> MTQVAKKILVTCALPYANGSIHLGHMLEHIQADVWVRYQRMRGHEVNFICADDAHGTPIMLKAQQLGITPEQMIGEMSQEHQTDFAGFNISYDNYHSTHSEENRQLSELIYSRLKENGFIKNRTISQLYDPEKGMFLPDRFVKGTCPKCKSPDQYGDNCEVCGATYSPTELIEPKSVVSGATPVMRDSEHFFFDLPSFSEMLQAWTRSGALQEQVANKMQEWFESGLQQWDISRDAPYFGFEIPNAPGKYFYVWLDAPIGYMGSFKNLCDKRGDSVSFDEYWKKDSTAELYHFIGKDIVYFHSLFWPAMLEGSNFRKPSNLFVHGYVTVNGAKMSKSRGTFIKASTWLNHFDADSLRYYYTAKLSSRIDDIDLNLEDFVQRVNADIVNKVVNLASRNAGFINKRFDGVLASELADPQLYKT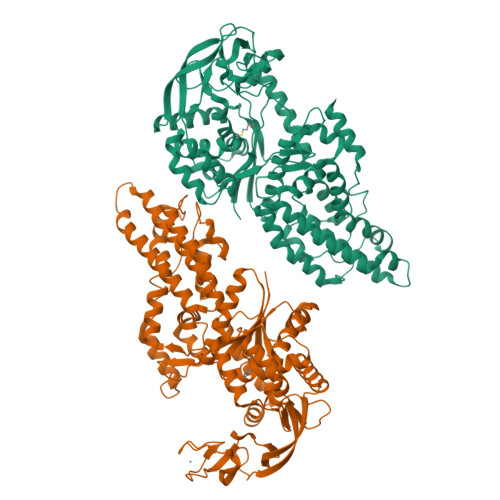FTDAAEVIGEAWESREFGKAVREIMALADLANRYVDEQAPWVVAKQEGRDADLQAICSMGINLFRVLMTYLKPVLPKLTERAEAFLNTELTWDGIQQPLLGHKVNPFKALYNRIDMRQVEALVEASKEEV>[3x]MA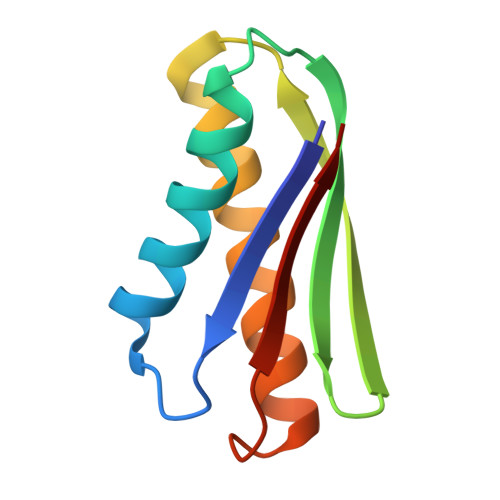SAEAEVKPDATIEEIRAAARRLAEALRKAGVSGPVTVTAEAGDVSFSYTADLDGTEEGLKRVVEAIVRAAIAALKATGGTKPVLLSAVLE>[2x]MAHHHHHHMKDHTIPLTLISILADGEFHSGEQLGEQLGMSRAAINKHIQTLRDWGVDVFTVPGKGYSLPEPIHLLDEKKISQEIDHGRVTVLPVIDSTNQYLLDRLDELTSGDACVAEYQQAGRGRRGRKWFSPFGANL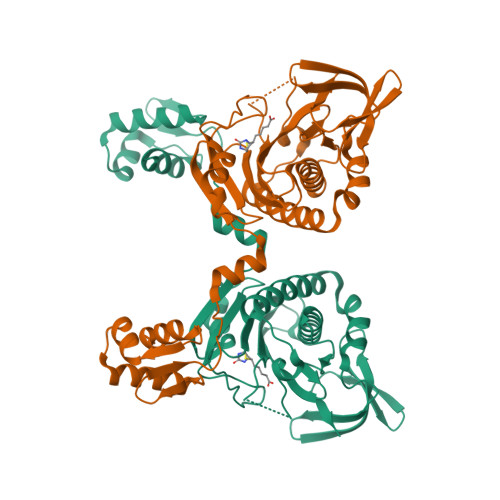YLSMYWRLEQGPAAAIGLSLVIGIVIAEVLQQLGAEQVRVKWPNDIYLQDRKLSGILVELTGKTGDAAQIVSGAGINLVMRRVESDVVNQGWISLQEAGVVIDRNLLAARLIKELRLGLELFEQEGLAPYLPRWEKLDNFIHRPVKLIIGDKEIYGISRGIDAQGALLLEQDGVIKAWVGGEISLRSAE> MASDYKDDDDKGALEVLFQGPSSPMAGNLVSWACKLCRSPEGFGPISFYGDFTQCFIDGVILNLSAIFMITFGIRDLVNLCKKKHSGIKYRRNWIIVSRMALVLLEIAFVSLASLNISKEEAENFTIVSQYASTMLSLFVALALHWIEYDRSVVANTVLLFYWLFETFGNFAKLINILIRHTYEGIWYSGQTGFILTLFQVITCASILLLEALPKKPLMPHQHIHQTLTRRKPNPYDSANIFSRITFSWMSGLMKTGYEKYLVEADLYKLPRNFSSEELSQKLEKNWENELKQKSNPSLSWAICRTFGSKMLLAAFFKAIHDVLAFTQPQLLRILIKFVTDYNSERQDDHSSLQGFENNHPQKLPIVRGFLIAFAMFLVGFTQTSVLHQYFLNVFNTGMYIKSALTALIYQKSLVLSNEASGLSSTGDIVNLMSVDVQKLQDLTQWLNLIWSGPFQIIICLYSLYKLLGNSMWVGVIILVIMMPLNSFLMRIQKKLQKSQMKYKDERTRVISEILNNIKSLKLYAWEKPYREKLEEVRNNKELKNLTKLGCYMAVTSFQFNIVPFLVSCCTFAVFVYTEDRALTTDLVFPALTLFNLLSFPLMIIPMVLNSFIEASVSIGRLFTFFTNEELQPDSVQRLPKVKNIGDVAINIGDDATFLWQRKPEYKVALKNINFQAKKGNLTCIVGKVGSGKTALLSCMLGDLFRVKGFATVHGSVAYVSQVPWIMNGTVKENILFGHRYDAEFYEKTIKACALTIDLAILMDGDKTLVGEKGISLSGGQKARLSLARAVYARADTYLLDDPLAAVDEHVARHLIEHVLGPNGLLHTKTKVLATNKVSALSIADSIALLDNGEITQQGTYDEITKDADSPLWKLLNNYGKKNNGKSNEFGDSSESSVRESSIPVEGELEQLQKLNDLDFGNSDAISLRRASDATLGSIDFGDDENIAKREHREQGKVKWNIYLEYAKACNPKSVCVFILFIVISMFLSVMGNVWLKHWSEVNSRYGSNPNAARYLAIYFALGIGSALATLIQTIVLWVFCTIHASKYLHNLMTNSVLRAPMTFFETTPIGRILNRFSNDIYKVDALLGRTFSQFFVNAVKVTFTITVICATTWQFIFIIIPLSVFYIYYQQYYLRTSRELRRLDSITRSPIYSHFQETLGGLATVRGYSQQKRFSHINQCRIDNNMSAFYPSINANRWLAYRLELIGSIIILGAATLSVFRLKQGTLTAGMVGLSLSYALQITQTLNWIVRMTVEVETNIVSVERIKEYADLKSEAPLIVEGHRPPKEWPSQGDIKFNNYSTRYRPELDLVLKHINIHIKPNEKVGIVGRTGAGKSSLTLALFRMIEASEGNIVIDNIAINEIGLYDLRHKLSIIPQDSQVFEGTVRENIDPINQYTDEAIWRALELSHLKEHVLSMSNDGLDAQLTEGGGNLSVGQRQLLCLARAMLVPSKILVLDQATAAVDVETDKVVQETIRTAFKDRTILTIAHRLNTIMDSDRIIVLDNGKVAEFDSPGQLLSDNKSLFYSLCMEAGLVNENGLVPRGSSAHHHHHHHHHHGA

Yeast Cadmium Factor 1 (Ycf1) belongs to the ATP Binding Cassette (ABC) transporter family and sequesters glutathione and glutathione heavy metal conjugates to the vacuole to detoxify reactive oxygen species and heavy metals (Cd2+, Se2+, Hg2+, As2+). Ycf1 belongs to the C subfamily (termed ABCC), which, in addition to the core architecture, includes several evolutionary additions, including an additional TMD (called TMD0), a lasso domain that links TMD0 and TMD1, and a flexible linker domain called the regulatory domain (R-domain) that connects NBD1 and TMD2. R-domain phosphorylation is necessary for activity, whereas dephosphorylation induces autoinhibition through an undefined mechanism.

Here, we sought to determine the structural changes in the dephosphorylated Ycf1 E1435Q mutant, expressed and purified from the Saccharomyces cerevisiae DSY5 strain. Surprisingly, dephosphorylation of Ycf1 leads to a complete loss of the R-domain density at its interaction site on NBD1 previously observed in the phosphorylated structures. Instead, considerable additional electron potential density was visible within the substrate-binding cavity between TMD1 and TMD2. This density displayed several continuous segments that allowed for the structural assignment of the C-terminal half of the R-domain (residues 890-935) continuous with TMD2 (see Methods for details of structure assignment). Apart from the substantive gross R domain rearrangement, the dephosphorylated Ycf1 architecture remains almost unchanged from the IFwide conformation of phosphorylated Ycf1. At this site, it adopts an unexpected helix-strand hairpin motif constructed of an α-helix (residues 902-912) with pronounced corresponding density in the cryo-EM map. This region encompasses three primary phosphorylation sites on Ycf1 (S903, S908, T911), including the RRAS motif. In conclusion, our dephosphorylated Ycf1 structure shows a dramatic rearrangement of the R-domain that occludes the transporter substrate binding pocket, resembling the peptide-bound state of TAP1/TAP2.>[3x]MFAIFVSSGSIKNDLNNLGEDMRFNQWMTCITSGLILASNSSFATTSPVHEQLQVPQCLAAKITVPHKILAENKEFKIIDVLSSDVETLTILADKVSCGHFVNVSHKLTGTLAANQQQSAQKLLQKKLVKPFGVSKLHKDVYEIKHEEEVNAALKEIVSDNIWQTLTHMTSYYNRSATKDTGVDTANWLKSKFEQMAVEYGRTDTSTFFVKTGWYKQPSLV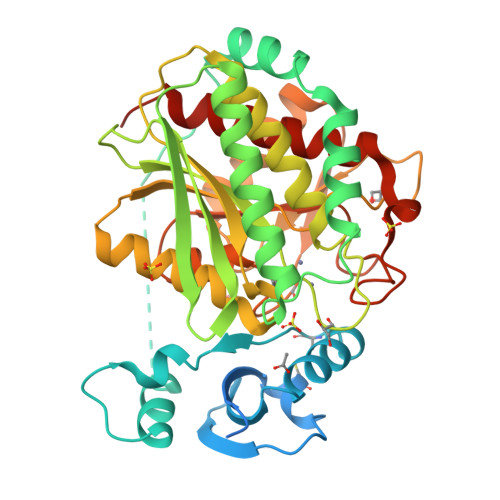TVIGKDIKAPAIVIGAHMDTLDGRMPGAGDDGSGSSSIMEAARVILSSKTTFKRPIYFIWYAAEERGLVGSQHVVQHFQEQSIPVKAVVQFDMTGYRNDANDPTMWVFTDYTDRDLSNYLAKLIDHYIHVPVDYSRCGYGCSDHASWNEEDIPAAFPCETSFADHNPYIHTSSDKMDLLNLEHMTNFSKLAVAFAIELASELEHHHHHH> AQSVPWGISRVQAPAA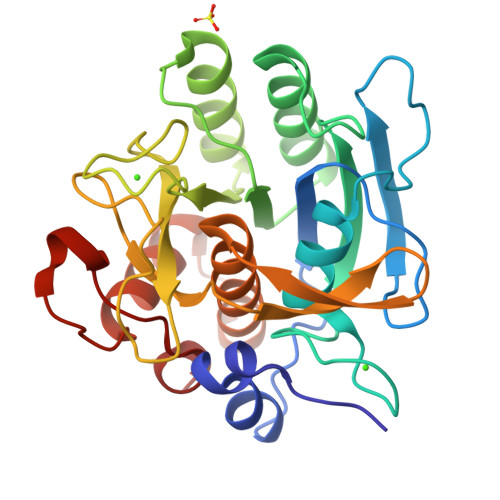HNRGLTGSGVRVAVLDTGISTHPDLNIRGGASFVPGEPSTQDGNGHGTHVAGTIAALNNSIGVLGVAPSAELYAVKVLGASGSGSYSSIAQGLEWAGNNGMHVASLSLGSPSPSATLEQAVNSATSRGVLVVAASGNSGAGSISYPARYANAMAVGATDQNNNRASFSQYGAGLDIVAPGVNVQSTYPGSTYASLNGTSMATPHVAGAAALVKQKNPSWSNVQIRNHLKNTATSLGSTNLYGSGLVNAEAAAR>[3x]EREKLLRLEEELHKRVVGQDEAIRAVADAIRRARAGLKDPNRPIGSFLFLGPTGVGKTELAKTLAATLFDTEEAMIRIDMTEYMEKHAVSRL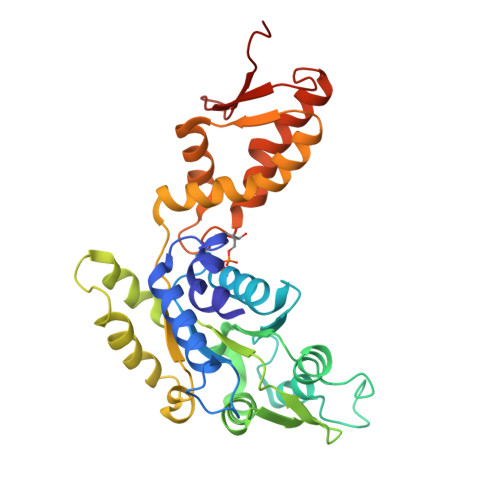IGAPPGYVGYEEGGQLTEAVRRRPYSVILFDAIEKAHPDVFNILLQILDDGRLTDSHGRTVDFRNTVIILTSNLGSPLILEGLQKGWPYERIRDEVFKVLQQHFRPEFLNRLDEIVVFRPLTKEQIRQIVEIQLSYLRARLAEKRISLELTEAAKDFLAERGYDPVFGARPLRRVIQRELETPLAQKILAGEVKEGDRVQVDVGPAGLVFAVPARV>GEFNTIQQLMMILNSASDQPSENLISYFNNCTVNPKESILKRVKDIGYIFKEKFAKAVGQGCVEIGSQRYKLGVRLYYRVMESMLKSEEERLSIQNFSKLLNDNIFHMSLLACALEVVMATYSRSTSQNLDSGTDLSFPWILNVLNLKAFDFYKVIESFIKAEGNLTREMIKHLERCEHRIMESLAWLSDSPLFDLIKQSKLVPRGSKSTSLSLFYKKVYRLAYLRLNTLCERLLSEHPELEHIIWTLFQHTLQNEYELMRDRHLDQIMMCSMYGICKVKNIDLKFKIIVTAYKDLPHAVQETFKRVLIKEEEYDSIIVFY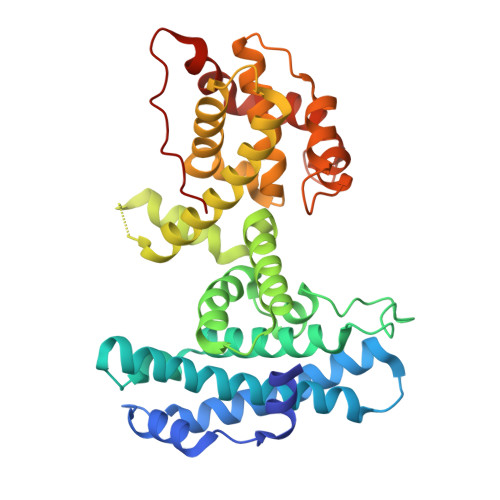NSVFMQRLKTNILQYASTRPPTLSPIPHIPR[2x]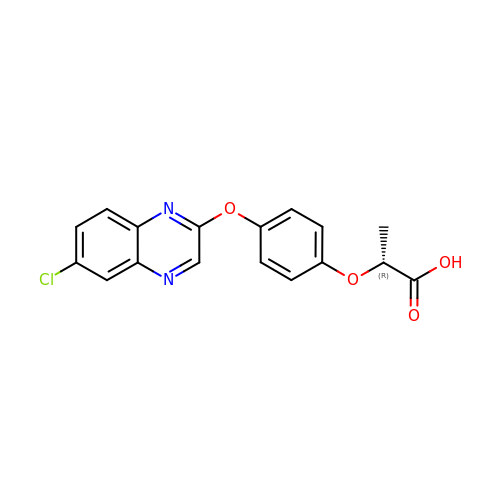(2R)-2-{4-[(6-chloroquinoxalin-2-yl)oxy]phenoxy}propanoic acid | C17 H13 Cl N2 O4 | ABOOPXYCKNFDNJ-SNVBAGLBSA-N>HMAHHHHHHMGFLDGKRILLTGLLSNRSIAYGIAKACKREGAELAFTYVGDRFKDRITEFAAEFGSELVFPCDVADDAQIDALFASLKTHWDSLDGLVHSIGFAPREAIAGDFLDGL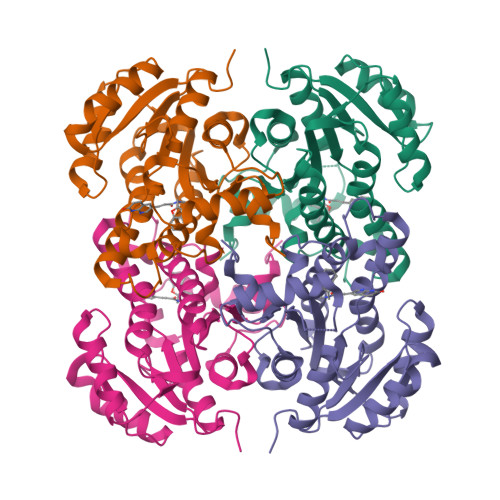TRENFRIAHDISAYSFPALAKAALPMLSDDASLLTLSYLGAERAIPNYNTMGLAKAALEASVRYLAVSLGAKGVRVNAISAGPIKTLAASGIKSFGKILDFVESNSPLKRNVTIEQVGNAGAFLLSDLASGVTAEVMHVDSGFNAVVGGMAGLEE[4x]>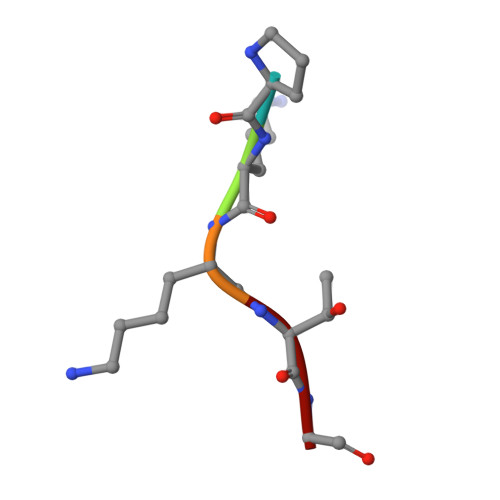 PKKTG>MATLVVNKLGAGVDSGRQGSRGTAVVKVLECGVCEDVFSLQGDKVPRLLLCGHTVCHDCLTRLPLHGRAIRCPFDRQVTDLGDSGVWG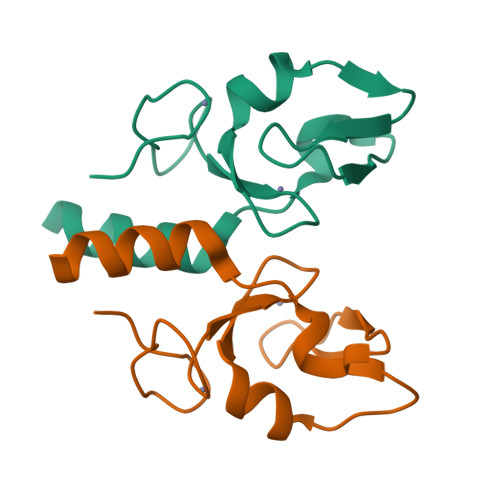LKKNFALLELLERLQNGPIGQYGAAEESIGISGES[3x]> SAVKAARYGKDNVRVYKVHKDEKTGVQTVYEMTVCVLLEGEIETSYTKADNSVIVATDSIKNTIYITAKQNPVTPPELFGSILGTHFIEKYN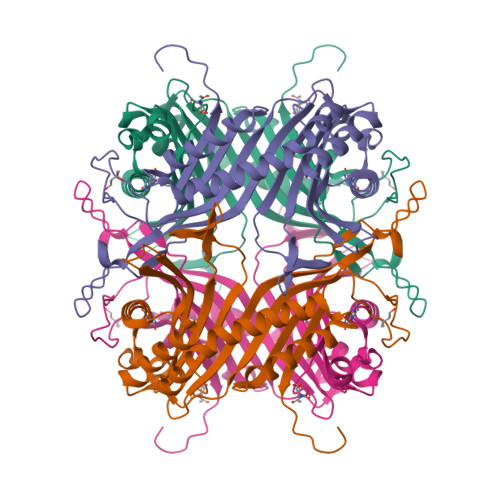HIHAAHVNIVCHRWTRMDIDGKPHPHSFIRDSEEKRNVQVDVVEGKGIDIKSSLSGLTVLKSTNSQFWGFLRDEYTTLKETWDRILSTDVDATWQWKNFSGLQEVRSHVPKFDATWATAREVTLKTFAEDNSASVQATMYKMAEQILARQQLIETVEYSLPNKHYFEIDLSWHKGLQNTGKNAEVFAPQSDPNGLIKCTVGRSSLKSKL> MAYKPQFYPGETKIAQNRRNHMNPEVELEKLREIPDEDVVKIMGHRQPGEDYKTIHPPLEEMDLPDDYVRDLVEPINGAKEGHRIRYIQFADSMYFAPAQPYDRARTYMWRFRGVDTGTLSGRQVIEMRESDLEALSKNFLIDTAFFDPARCGIRGATVHGHSLRLDENGLMFDALQR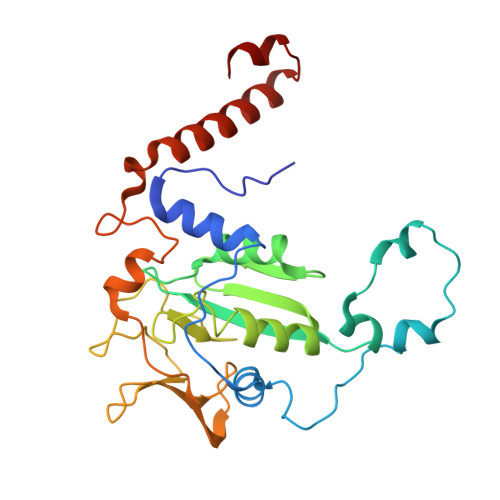YVYDEKTGHVVYVKDQVGRPLDEPVDVGELLPEEKLREITTIYRKDGVPMREDKELLTIVKRIHRARTLGGFCPTEDTFKQL Repaglinide | C27 H36 N2 O4 | 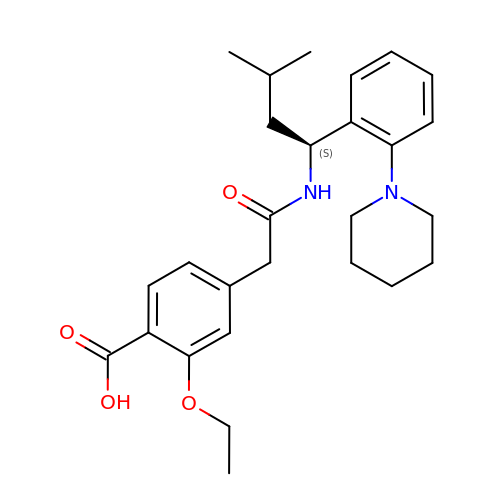FAEKWTJYAYMJKF-QHCPKHFHSA-N> REWWSE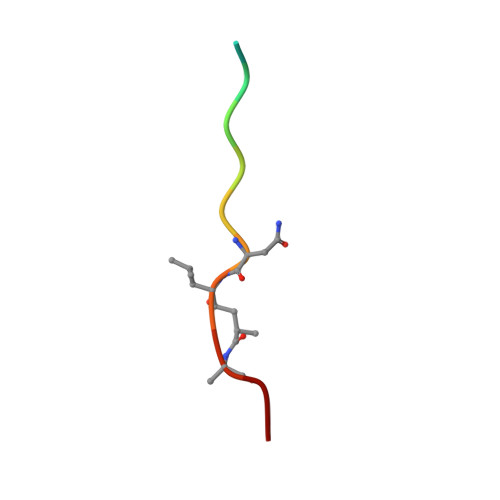VNXAEF4-(4-methyl-1~{H}-imidazol-5-yl)-~{N}-(4-morpholin-4-ylphenyl)pyridin-2-amine | C19 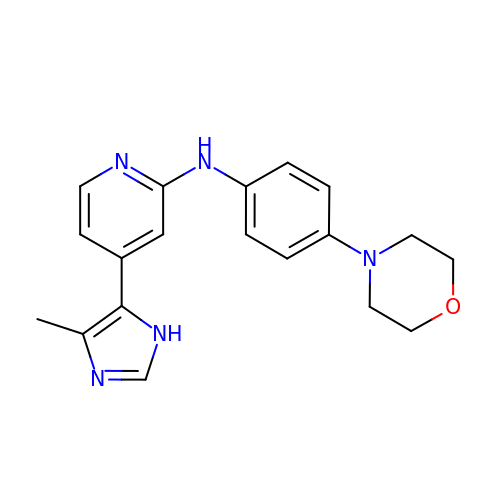H21 N5 O | KJQAULYFYNEAHK-UHFFFAOYSA-N> MGSSHHHHHHSSGLVPRGSHSDEVDAHMTTNTVSRKVAWLRVVTLAVAAFIFNTTEFVPVGLLSDIAQSFHMQTAQVGIMLTIYAWVVALMSLPFMLMTSQVERRKLLICLFVVFIASHVLSFLSWSFTVLVISRIGVAFAHAIFWSITASLAIRMAPAGKRAQALSLIATGTALAMVLGLPLGRIVGQYFGWRMTFFAIGIGALITLLCLIKLLPLLPSEHSGSLKSLPLLFRRPALMSIYLLTVVVVTAHYTAYSYIEPFVQNIAGFSANFATALLLLLGGAGIIGSVIFGKLGNQYASALVSTAIALLLVCLALLLPAANSEIHLGVLSIFWGIAMMIIGLGMQVKVLALA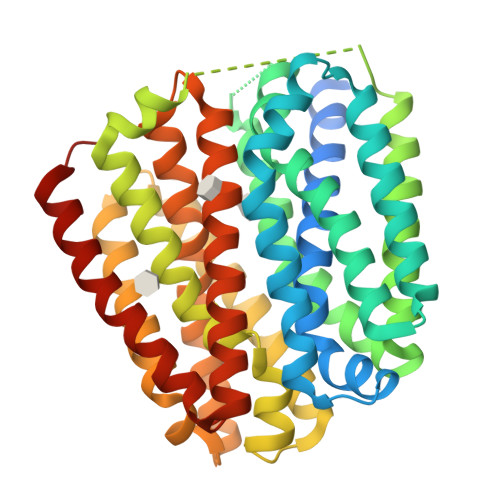PDATDVAMALFSGIFNIGIGAGALVGNQVSLHWSMSMIGYVGAVPAFAALIWSIIIFRRWPVTLEEQTQ>[2x]DVQTALQHSIREIGLRLMRMKNDGMSQKDIAAK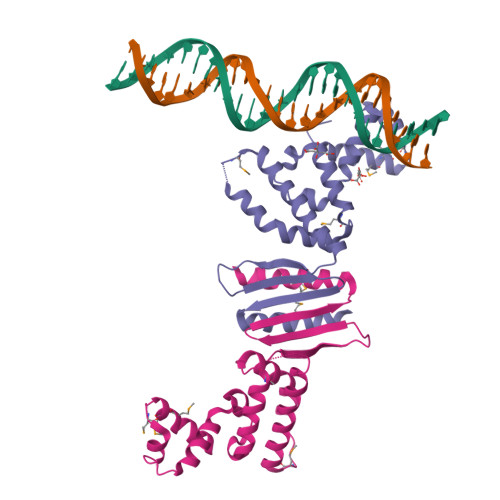EGLSQAKVTRALQAASAPEELVALFPVQSELTFSDYKTLCAVGDEMGNKNLEFDQLIQNISPEINDILSINEMAEDEVKNKILRLITKEASLLTDKGSKDKSVVTELWKFEDKDRFARKRVKGRAFSYEFNRLSKELQEELDRMIGHILRKSLDKKPKP> MKYQQLENLECGWKWAY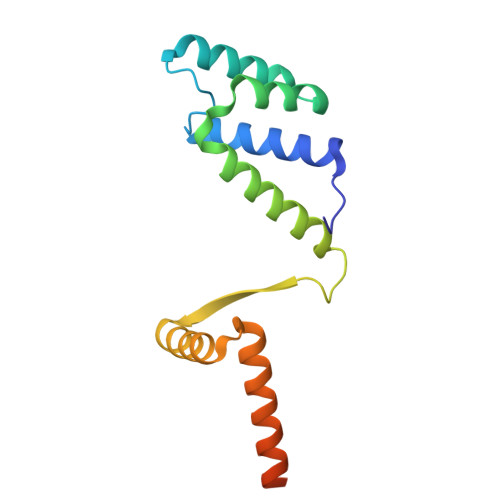LIRKHQEGEPITKYIENSAAHAAVDKLIKLESEPVRVLEWIEQHMNPDLFNRMKQTIRARRKRHFNAEHQHTRKKSIDLDFPVWHRLSALSQRRGNTLSETIVQLIEDAERKEKYANQMSSLKHDLEAILGKNE> YLDDFENWTVVPVETIEGINYYPNCLPESVQRNLINNVPKELLSIYGSGKQSHLYIPFPAHINCLNDYIPSDFKQRLWKGQ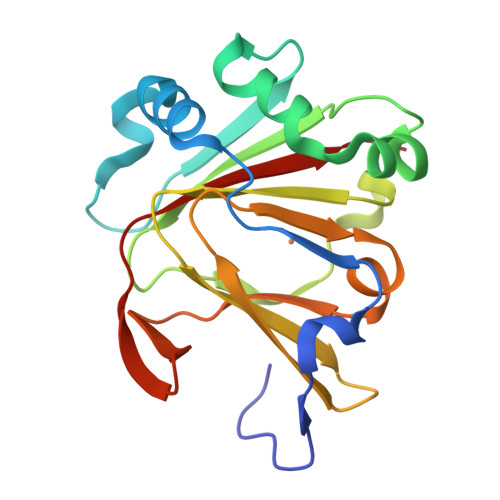DAEAIIMQVYNPGDGIIPHKDLEMFGDGVAIFSFLSNTTMIFTHPELKLKSKIRLEKGSLLLMSGTARYDWFHEIPFRAGDWVMNDGEEKWVSRSQRLSVTMRRII>GPLGSPVVVRGWLHKQKSSGMRLWKRRWFVLADYCLFYYKDSREEAVLGSIPLPSYVISPVAPEDRISRKYSFKAVHTGMRALIYNSSTAGSQAEQSGMRTYYFSADTQEDM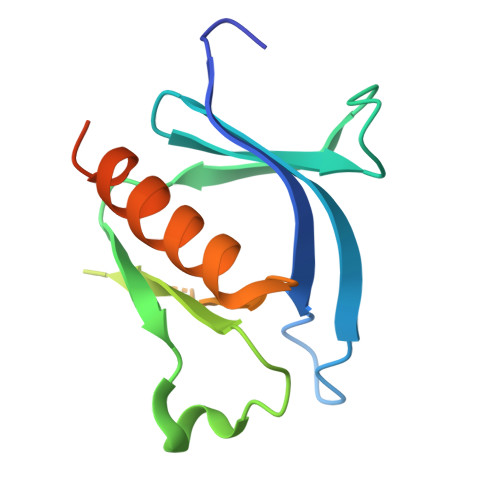NAWVRAMNQAAQVLSRSSLKRDMEKVER[2x]>[2x]GAHMVTSNVVLVSGEGERFTVDKKIAERSLLLKNYLNDMGDDDDEDD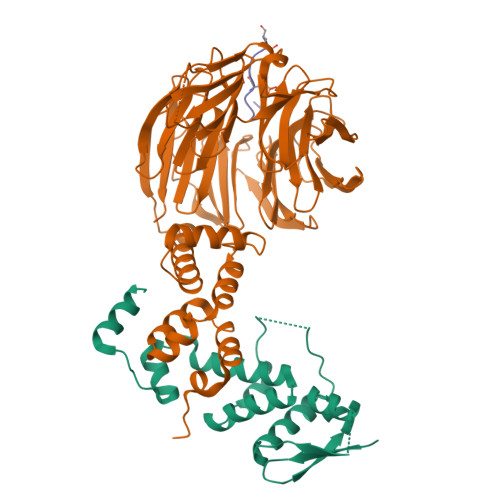DEIVMPVPNVRSSVLQKVIEWAEHHRDSNFPDEDDDDSRKSAPVDSWDREFLKVDQEMLYEIILAANYLNIKPLLDAGCKVVAEMIRGRSPEEIRRTFNIVNDFTPEEEAAIRRENEWAEDR;>GAGTLIKDNLKRDLITSLPFEISLKIFNYLQFEDIINSLGVSQNWNKIIRKSTSLWKKLLISENFVSPKGFNSLNLKLSQKYPKLSQQDRLRLSFLENIFILKNWYNPKFVPQRTTLRGHMTSVITCLQFEDNYVITGADDKMIRVYDSINKKFLLQLSGHDGGVWALKYAHGGILVSGSTDRTVRVWDIKKGCCTHVFEGHNSTVRCLDIVEYKNIKYIVTGSRDNTLHVWKLPKESSVPDHGEEHDYPLVFHTPEENPYFVGVLRGHMASVRTVSGHGNIVVSGSYDNTLIVWDVAQMKCLYILSGHTDRIYSTIYDHERKRCISASMDTTIRIWDLENGELMYTLQGHTALVGLLRLSDKFLVSAAADGSIRGWDANDYSRKFSYHHTNLSAITTFYVSDNILVSGSENQFNIYNLRSGKLVHANILKDADQIWSVNFKGKTLVAAVEKDGQSFLEILDFS[2x];> MTSPFNGLTSPQRSPFPKS5-{[5-(6-aminopyridin-2-yl)-2-chlorobenzene-1-carbonyl]amino}-1-phenyl-1H-pyrazole-3-carboxamide | C22 H17 Cl N6 O2 | 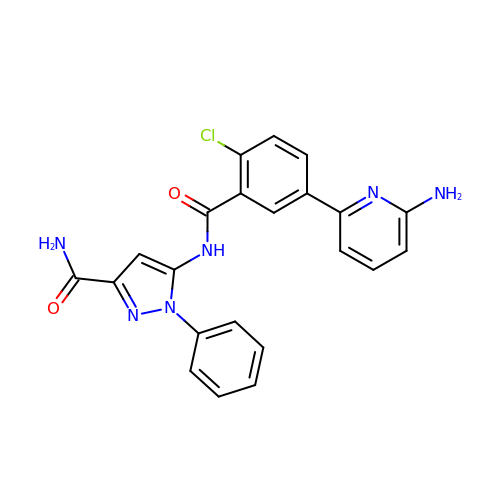YVUMGRGBUXDTQI-UHFFFAOYSA-N(S)-2-(8-(2-Amino-4-oxo-4,7-dihydro-3H-pyrrolo[2,3-d]pyrimidin-6-yl)octanamido)pentanedioic 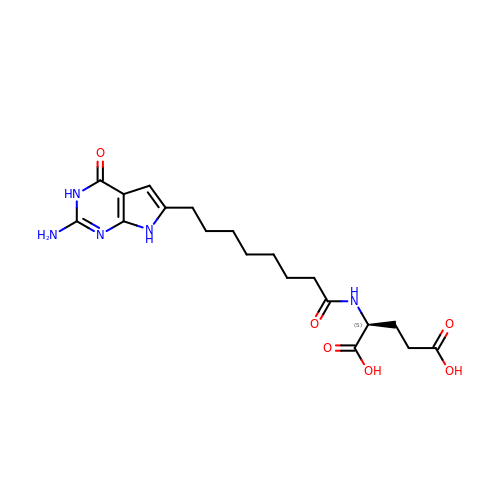acid | C19 H27 N5 O6 | MZFFIVGWDCAMQT-ZDUSSCGKSA-N> GSQDLSDSYERLNNLLTNYSVLNALIRQSADPNAINNARGNLNASAKNLINDKKNSPAYQAVLLALNAAAGLWQVMSYAISPCGPGKDTSKNGGVQTFHNTPSNQWGGTTITCGTTGYEPGPYSILSTENYAKINKAYQIIQKAFGSSGKDIPALSDTNTELKFTINKNNGNTNTNNNGEEIVTKNNAQVLL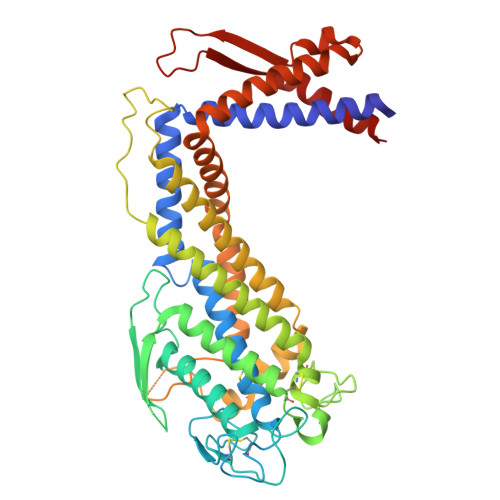EQASTIITTLNSACPWINNGGAGGASSGSLWEGIYLKGDGSACGIFKNEISAIQDMIKNAAIAVEQSKIVAANAQNQRNLDTGKTFNPYKDANFAQSMFANAKAQAEILNRAQAVVKDFERIPAEFVKDSLGVCHEVQNGHLRGTPSGTVTDNTWGAGCAYVGETVTNLKDSIAHFGDQAERIHNARNLAYTLANFSSQYQKLGEHYDSITAAISSLPDAQSLQNVVSKKTNPNSPQGIQDNYYIDSNIHSQVQSRSQELKGS>[2x]GMGGRRTIGIRSGEGAIMNASDFYALLRGRGMPVVVDDAEAAAVVSELGFRTVPFEAFDFDSPSEDPALVIVAQMGNVDALHGLWERSGTPLMHLALAKFDGGLSRLRAGLARVLAVDTDAALKRRAEAYEQLFSSASVEIASGEGVLRCHIGDEVEVGNCGDTLEQGFLYSVAEFLEASVVNLEGER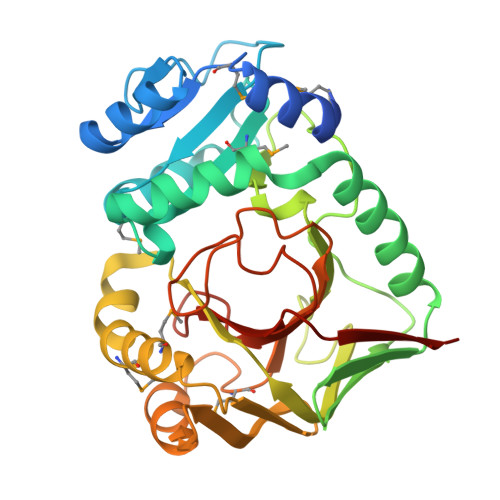STFWVEGELPFDGFIHLSNSAALKERWGGMLDEFMRRSREGANLVRFADNVIDRLVVGGVDVTSALAGLSQGEERGMAATEFGLGCADAEAAEPFGVNSLLHKSAGGAYIGIGKGLRIPHIDFIARGATIRFIPAAEG2-(morpholin-4-ium-4-ylmethyl)naphthalen-1-ol | C15 H18 N O2 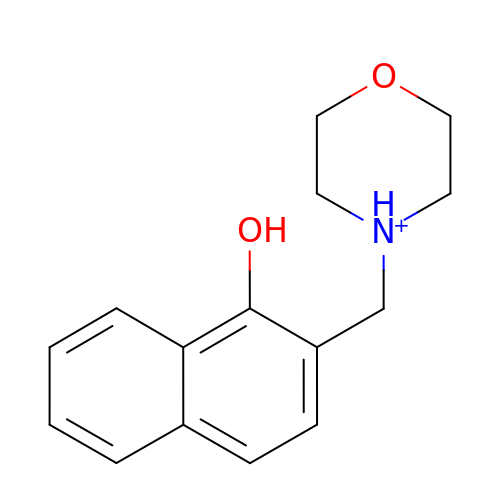| XJKMEOFFCYJCGT-UHFFFAOYSA-O>[2x]MSNKCDVVVVGGGISGMAAAKLLHDSGLNVVVLEARDRVGGRTYTLRNQKVKYVDLGGSYVGPTQNRILRLAKELGLETYKVNEVERLIHHVKGKSYPFRGPFPPVWNPITYLDHNNFWRTMDDMGREIPSDAPWKAPLAEEWDNMTMKELLDKLCWTESAKQLATLFVNLCVTAETHEVSALWFLWYVKQCGGTTRIISTTNGGQERKFVGGSGQVSERIMDLLGDRVKLERPVIYIDQTRENVLVETLNHEMYEAKYVISAIPPTLGMKIHFNPPLPMMRNQMITRVPLGSVIKCIVYYKEPFWRKKDYCGTMIIDGEEAPVAYTLDDTKPEGNYAAIMGFILAHKARKLARLTKEERLKKLCELYAKVLGSLEALEPVHYEEKNWCEEQYSGGCYTTYFPPGILTQYGRVLRQPVDRIYFAGTET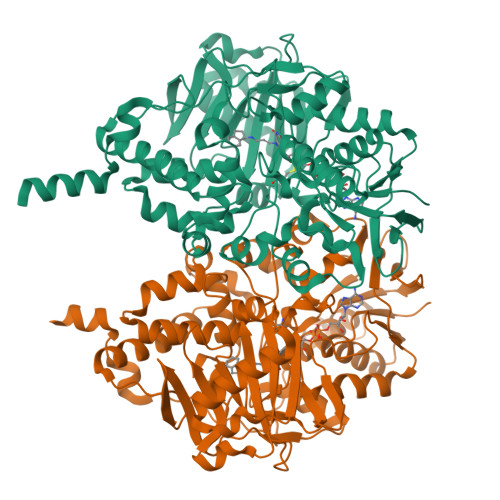ATHWSGWMEGAVEAGERAAREILHAMGKIPEDEIWQSEPESVDVPAQPITTTFLERHLPSVPGLLRLIGLTTIFSATALGFLAHKRGLLVRV> MVQRWLYSTNAKDIAVLYFMLAIFSGMAGTAMSLIIRLELAAPGSQYLHGNSQLFNVLVVGHAVLMIFFLVMPALIGGFGNYLLPLMIGATDTAFPRINNIAFWVLPMGLVCLVTSTLVESGAGTGWTVYPPLSSIQAHSGPSVDLAIFALHLTSISSLLGAINFIVTTLNMRTNGMTMHKLPLFVWSIFITAFLLLLSLPVLSAGITMLLLDRNFNTSFFEVSGGGDPILYEHLFWFFGHPEVYILIIPGFGIISHVVSTYSKKPVFGEISMVYAMASIGLLGFLVWSHHMYIVGLDADTRAYFTSATMIIAIPTGIKIFSWLATIHGGSIRLATPMLYAIAFLFLFTMGGLTGVALANASLDVAFHDTYYVVGHFHYVLSMGAIFSLFAGYYYWSPQILGLNYNEKLAQIQFWLIFIGANVIFFPMHFLGINGMPRRIPDYPDAFAGWNYVASIGSFIATLSLFLFIYILYDQLVNGLNNKVNNKSVI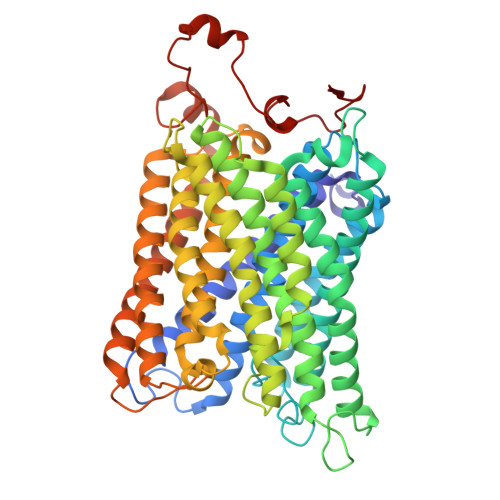YNKAPDFVESNTIFNLNTVKSSSIEFLLTSPPAVHSFNTPAVQS>QQASTLPDLAEQFAPPDVAPPLLIKLVKAIEKKGLECSTLYRTQSSSNPAELRQLLDCDTASLDLEMFDVHVLADAFKRYLLDLPNPVIPVAVSSELISLAPEVQSSEEYIQLLKKLIRSPSIPHQYWLTLQYLLKHFFKLSQTSSKNLLNARVLSELFSPLLFRFPAASSENTEHLIKIIEILISTEWNERQ[2x]

The N-terminal domains of p85α include an SH3 domain, capable of binding to proline-rich sequences, and a BH (breakpoint cluster region homology) domain. The BH domain can bind to and regulate several GTPases including Rab5, Rac1 and Cdc42. In addition, the p85α BH domain, either alone or together with the SH3 domain, can bind to and positively regulate PTEN activity. The p85α BH domain also exhibits Rab5 GAP activity to stimulate Rab5-mediated GTP hydrolysis required to inactivate Rab5-mediated protein trafficking functions.

To determine if the patient-derived p85α BH domain mutations impacted the overall folded structure of the BH domain, several of these BH domain mutants were crystalized and their structures were determined using X-ray crystallography. X-ray diffraction data collection and structure refinement statistics for bovine p85α (105–319) mutants (E137K, E217K, R262T, E297K) are provided in Supplementary Table S1. In contrast, several of the p85α mutants (E137K, K288Q, E297K) showed near wild type binding to PTEN, and either had enhanced (K288Q) or reduced (E297K, E137K) ability to stimulate PTEN lipid phosphatase activity. Three BH domain mutants, I177N, E217K and E297K, all showed significantly increased Rab5-GAP activity, whereas the E137K mutant had reduced activity. The location of cancer patient-derived p85α BH mutations with significant impacts on Rab5 binding (I177, E217) and/or regulation (E137, I177, E217, E297) are shown in the modeled p85α BH domain: Rab5 complex. These mutation sites are located in regions of the p85α BH domain, well away from the Rab5 binding pocket. Further, crystal structure determinations for several of these mutant BH domains indicated that no major structural alterations were present. No significant differences in protein flexibility were observed for any of the mutant proteins, suggesting that the mutations did not alter the rigidity of the domain.> MAHHHHHHLVPRGSHETEQSVDLETVSVVGKSRPRATSGLLHTSTASDKIISGDTLRQKAVNLGDALDGVPGIHASQYGGGASAPVIRGQTGRRIKVLNHHGETGDMADFSPDHAIMVDTALSQQVEILRGPVTLLYSSGNVAGLVDVADGKIPEKMPENGVSGELGLRLSSGNLEKLTSGGINIGLGKNFVLHTEGLYRKSGDYAVPRYRNLKRLPDSHADSQTGSIGLSWVGEKGFIGVAYSDRRDQYGLPAHSHEYD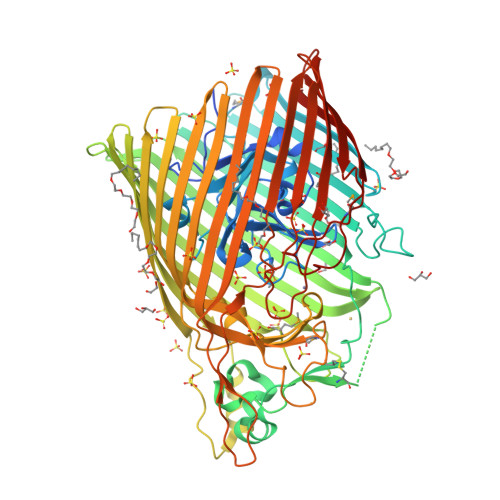DCHADIIWQKSLINKRYLQLYPHLLTEEDIDYDNPGLSCGFHDDDNAHAHTHSGRPWIDLRNKRYELRAEWKQPFPGFEALRVHLNRNDYRHDEKAGDAVENFFNNQTQNARIELRHQPIGRLKGSWGVQYLQQKSSALSAISEAVKQPMLLDNKVQHYSFFGVEQANWDNFTLEGGVRVEKQKASIQYDKALIDRENYYNHPLPDLGAHRQTARSFALSGNWYFTPQHKLSLTASHQERLPSTQELYAHGKHVATNTFEVGNKHLNKERSNNIELALGYEGDRWQYNLALYRNRFGNYIYAQTLNDGRGPKSIEDDSEMKLVRYNQSGADFYGAEGEIYFKPTPRYRIGVSGDYVRGRLKNLPSLPGREDAYGNRPFIAQDDQNAPRVPAARLGFHLKASLTDRIDANLDYYRVFAQNKLARYETRTPGHHMLNLGANYRRNTRYGEWNWYVKADNLLNQSVYAHSSFLSDTPQMGRSFTGGVNVKF> MAAALSEQLAELEKRSGGRLGVAVLDTATGRRFGYRGDERFPMCSTFKALLAAAVLARVDQGKENLDRRITYGKEDLVDYSPVTEKHVGDGMTVAELCEAAITYSDNTAANLLLEALGGPAALTAFLRSIGDNVTRLDRWEPELNTAAPGDPRDTTTPAAMAATLRTLLLGDVLSPASRQQLVDWLIANKTGDKRLRAGLPADDRVGDKTGTGEHGTTNDIAVIWPPNRAPILVAVYLTESQVDADARDAVIAEVARLVVAAWHHHHHH

Here, we explore and test these notions using resurrected Precambrian β-lactamases11 as scaffolds for the engineering of completely new active sites. Of these systems, resurrected Precambrian β-lactamases have been thoroughly characterized in terms of their structure, function and stability. These putative ancestral proteins have been shown to be highly stable and able to efficiently degrade several antibiotics. A hydrophobic-to-ionizable amino acid replacement generates a buried (or partially buried) residue with the perturbed properties that are useful in catalysis and conformational flexibility assists the generation of a completely new active site by facilitating substrate and transition-state binding. We have shown that, when using resurrected Precambrian β-lactamases as scaffolds for protein engineering, a minimalist design approach based on this mechanism leads to levels of catalysis for the Kemp elimination reaction of up to approximately seven orders of magnitude above the rate of the uncatalysed reaction, as well as to significant ester hydrolysis activity.

Finally, catalysis of Kemp elimination is enhanced by an additional F290W amino replacement in the neighbourhood of position 229, which likely stabilizes the transition state through a face-to-edge interaction with the new tryptophan residue. Furthermore, the double W229/F290W variant of the GNCA4 scaffold is the most active Kemp eliminase reported in this work with a rate enhancement of about seven orders of magnitude over the rate of the uncatalysed reaction. Regarding the turnover numbers, the kcat values obtained for the W229D/F290W variants of the ancestral β-lactamase scaffolds are up to approximately seven orders of magnitude above the rate of the uncatalysed reaction. Unlike previous rationally designed Kemp eliminases, our best eliminase displays a maximum catalytic efficiency (∼5, 500 M−1 s−1) that exceeds the acetate in acetonitrile level. We therefore determined the Michaelis–Menten parameters for the degradation of a penicillin antibiotic (benzylpenicillin) and one third-generation antibiotic (cefotaxime) catalysed by GNCA4-W229D/F290W. We found levels of catalysis for antibiotic degradation similar to those previously reported for the GNCAMP β-lactamase. Our results show that the GNCA4-W229D/F290W β-lactamase does in fact also catalyse the hydrolysis of p-nitrophenyl acetate, a substrate commonly used to assess esterase activity. The catalytic efficiency for the hydrolysis of p-nitrophenyl acetate at the new active site, kcat/KM=11.7±1.1 M−1 s−1, is similar to the best values reported in the literature for rationally designed esterases. Furthermore, the turnover number at the new active site, kcat=7.6 × 10−3±2 × 10−4 s−1, indicates a three orders of magnitude enhancement over the rate of the non-enzymatic reaction (kuncat=2.5 × 10−6 s−1).> MNLESLLHWIYVAGMTIGALHFWSLSRNPRGVPQYEYLVAMFIPIWSGLAYMAMAIDQGKVEAAGQIAHYARYIDWMVTTPLLLLSLSWTAMQFIKKDWTLIGFL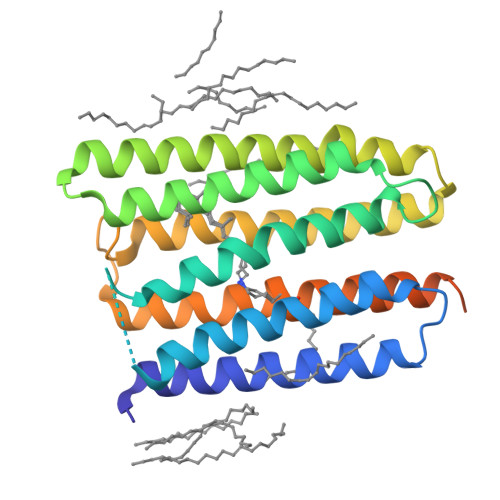MSTQIVVITSGLIADLSERDWVRYLWYICGVCAFLIILWGIWNPLRAKTRTQSSELANLYDKLVTYFTVLWIGYPIVWIIGPSGFGWINQTIDTFLFCLLPFFSKVGFSFLDLHGLRNLNDSRQTTGDRFAENTLQFVENITLFANSRRQQSRRRV The 2-HCT family of transporters generally translocate molecules with a 2-hydroxycarboxylate motif (HO-CR1R2-COO−), such as citrate, malate and lactate across the plasma membrane, and activity is tightly coupled to energy provided by a sodium or proton gradient as a form of secondary active transport. Our crystal structures reveal that the KpCitS protomer is formed by homologous N-terminal and C-terminal halves with inverted topology, each containing six transmembrane helices (TM 2–5, 7 and TM 8–11, 13) and one helical hairpin (TM 6a/b (or HP1) and TM 12a/b (or HP2)). KpCitS protomer can be divided into two domains; a central dimerization domain (TM 1–4 and 8–10) critical for formation of the dimeric structure, and a peripheral transport domain (TM 5–7 and 11–13) containing residues needed for interaction with citrate and sodium ions. Our results show that the KpCitS has a homodimeric structure in which its dimerization domain remains fixed during the transport cycle due to a hydrogen bond network as well as extensive hydrophobic interactions, while the substrate-loaded transport domain undergoes an elevator-type translocation (i.e. up and down) across the membrane.

Citrate-free KpCitS yielded a crystal diffracting to 3.6 Å resolution (form 3) with two inward-facing KpCitS dimers in an asymmetric unit. The dimers are practically identical, with Cα rms differences below 0.3 Å, suggesting that this state is structurally stable in the crystallization conditions. In the citrate-free inward-facing state, we observed that one water molecule takes the place of a citrate (right). Since the substrate binding site is continuous with the cytoplasm, water molecules are able to move deep into the membrane inner leaflet. In addition to the changes in amino acid conformation polar water molecules also seem to facilitate release of the substrate into the cell by breaking the electrostatic interactions between substrate and transporter. Conversely, D112, E195, R205 and Y348 form a salt bridge network in the inward-facing conformation, blocking entry of substrate from the periplasm. The conformational change to the inward-facing state relocates L408 and M417, opening the substrate binding site to the cytosol.

>[4x]GSKGVSDLLGFKIFGMPLPLYAFALITLLLSHFYNALPTDIVGGFAIMFIIGAIFGEIGKRLPIFNKYIGGAPVMIFLVAAYFVYAGIFTQKEIDAISNVMDKSNFLNLFIAVLITGAILSVNRRLLLKSLLGYIPTILMGIVGASIFGIAIGLVFGIPVDRIMMLYVLPIMGGGNGAGAVPLSEIYHSVTGRSREEYYSTAIAILTIANIFAIVFAAVLDIIGKKHTWLSGEGELVRKASFKVEEDEKTGQITHRETAVGLVLSTTCFLLAYVVAKKILPSIGGVAIHYFAWMVLIVAALNASGLCSPEIKAGAKRLSDFFSKQLLWVLMVGVGVCYTDLQEIINAITFANVVIAAIIVIGAVLGAAIGGWLMGFFPIESAITAGLCMANRGGSGDLEVLSACNRMNLISYAQISSRLGGGIVLVIASIVFGMMIPR Human thymidine phosphorylase (hTP, EC 2.4.2.4), identified as the sole endothelial mitogenic and angiogenic factor, belongs to the pyrimidine nucleoside phosphorylase (PyNP) family. Thymidine phosphorylase, providing pyrimidine nucleotides for DNA repair and replication, has also been shown to have angiogenic activity in vivo. Here, we report the crystal structures of recombinant native hTP and in complex with 5-iodouracil (5IUR), a substrate with a Ki of 0.48 mM. The active site is located at the interface between the α- and the mixed α/β-domain.

All four copies of hTP contain residues 34–479, residues 32 and 33 can be observed for chains A and B while only residue 33 can be observed for molecule C. At the C-terminal end, residue 480 was observed only in chain B. The crystal structure of hTP–5IUR complex (at 2.5 Å) consists of a dimer per asymmetric unit. Both chains comprise of residues 35–480 with one molecule of 5IUR bound in the active site of each hTP molecule. So far the two reported crystal structures of hTP were both in the closed form, based on which we can argue that binding of 5IUR in the active site of hTP leads to closed conformation. A total of six potential hydrogen bonds stabilize the binding of 5IUR in the active site of hTP. His116 directly interacts with 5IUR via its NE2 group. Almost opposite to His116 is Arg202, bonded via its amino groups to O4 of 5IUR. The other residues which are also involved in hydrogen-bonding interactions with 5IUR are Ser217 and Lys221. Eleven hTP residues are involved in potential van der Waals interactions with 5IUR have suggested that Val208 and Ile214 of the α-domain and Leu148 and Val241 of the α/β-domain stabilize the chlorine atom of TPI by forming a hydrophobic pocket. The iodine atom of 5IUR, appears to be similarly stabilized in the hydrophobic pocket. Apart from the residues that interact with 5IUR via hydrogen bonds, a hydrophobic pocket lined by Leu148, Val208, Ile214 and Val241, contributes to the stabilization of the molecule by holding the ‘iodine’ atom in place.

>[2x]MAALMTPGTGAPPAPGDFSGEGSQGLPDPSPEPKQLPELIRMKRDGGRLSEADIRGFVAAVVNGSAQGAQIGAMLMAIRLRGMDLEETSVLTQALAQSGQQLEWPEAWRQQLVDKHSTGGVGDKVSLVLAPALAACGCKVPMISGRGLGHTGGTLDKLESIPGFNVIQSPEQMQVLLDQAGCCIVGQSEQLVPADGILYAARDVTATVDSLPLITASILSKKLVEGLSALVVDVKFGGAAVFPNQEQARELAKTLVGVGASLGLRVAAALTAMDKPLGRCVGHALEVEEALLCMDGAGPPDLRDLVTTLGGALLWLSGHAGTQAQGAARVAAALDDGSALGRFERMLAAQGVDPGLARALCSGSPAERRQLLPRAREQEELLAPADGTVELVRALPLALVLHELGAGRSRAGEPLRLGVGAELLVDVGQRLRRGTPWLRVHRDGPALSGPQSRALQEALVLSDRAPFAAPSPFAELVLPPQQ> MGSSHHHHHHSQDPMAVRLVWSPTAKADLIDIYVMIGSENIRAADRYYDQLEARALQLADQPRMGVRRPDIRPSARMLVEAPFVLLYETVPDTDDGPV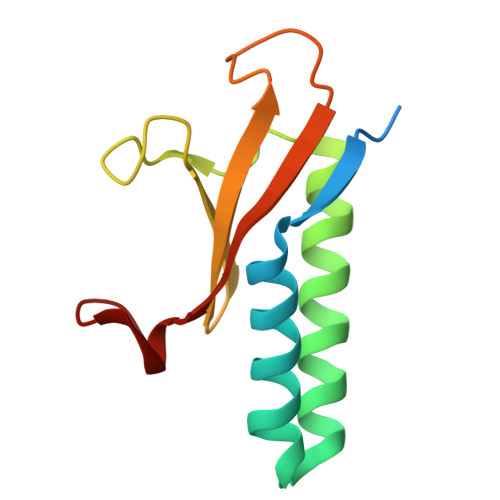EWVEIVRVVDGRRDLNRLF>SFKPTISVHATPQELSAAGCRKIVEIIEASGSQQWPLSIALAGGSTPKMTYARLHDEHLNLLREKRALRFFMGDERMVPADSTDSNYNMAREVLLHDIPDDLVFPFDTSAVTPSAEATSADAMRVAEAYGKQLASLLPLKSVGEAGPKVPVFDVVLLGLGSDGHTASIFPGSQA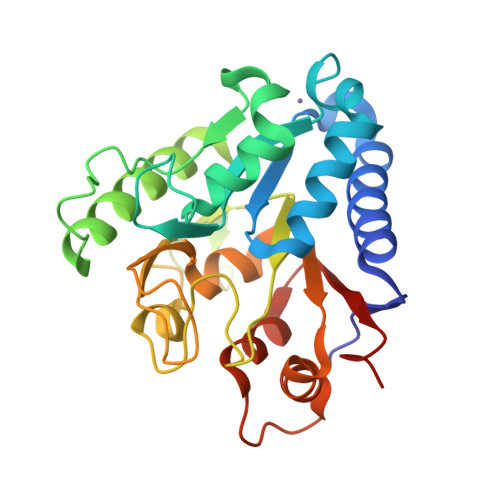EKETDGKVVVSVGFPSETMKPKVWRVTLSPATIMQARNVIVLATGAEKKWVVDGILADTAHKAPVARFLRGCEGNVSFLLDKEIAENLAKF[2x]>VETISFSFSEFEPGNNDLTLQGAAIITQSGVLQLTKINQNGMPAWDSTGRTLYTKPVHIWDMTTGTVASFETRFSFSIEQPYTRPLPADGLVFFMGPTKSKPAQGYGYLGVFNNSKQDNSYQTLAVEFDTFSNPWDPPQVPHIGIDVNSIRSIKTQPFQLDNGQVANVVIKYDASSKILLAVLVYPSSGAIYTIAEIVDVKQVLPEWVDVGLSGATGAQRDAAETHDVYSWSFHASLPETND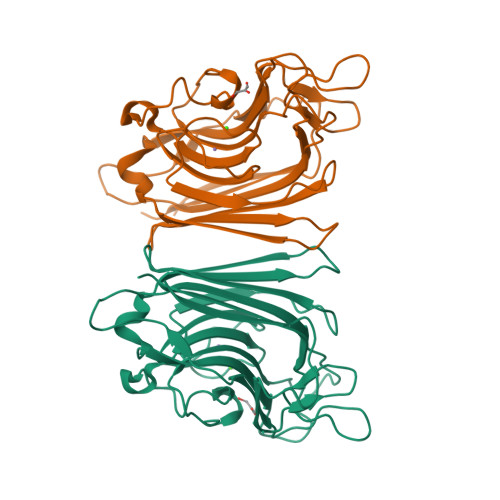[4x]(2S)-3-(carbamoylamino)-2-methylpropanoic 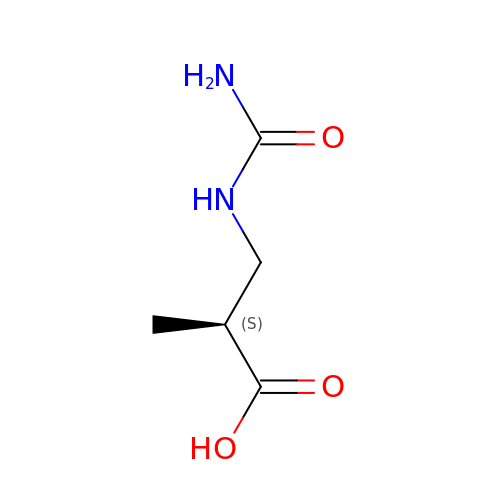acid | C5 H10 N2 O3 | PHENTZNALBMCQD-VKHMYHEASA-N N~2~-[(4-fluoro-3-methylphenyl)sulfonyl]-N-hydroxy-N~2~-(2-methylpropyl)-D-valinamide 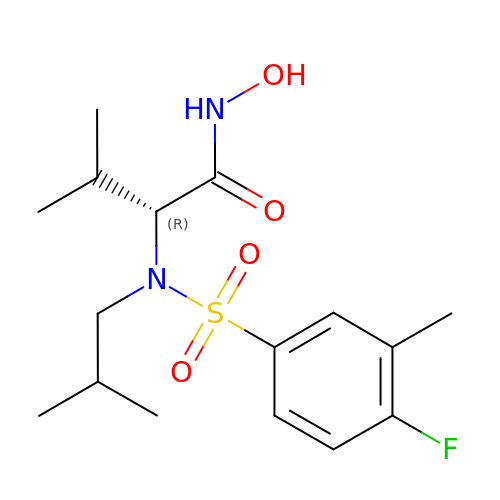| C16 H25 F N2 O4 S | XENBIBQWLKQPNV-OAHLLOKOSA-N> GMLASQQNQ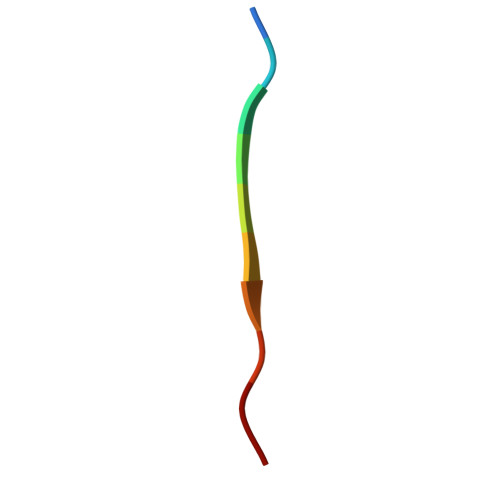S>GHHHHHHHHHHSSGHIEGRHMRVLFVSSPGIGHLFPLIQLAWGFRTAGHDVLIAVAEHADRAAAAGLEVVDVAPDYSAVKVFEQVAKDNPRFAETVATRPAIDLEEWGVQIAAVNRPLVDGTMALVDDYRPDLVVYEQGATVGLLAADRAGVPAVQRNQSAWRTRGMHRSIASFLTDLMDKHQVSLPEPVATIESFPPSLLLEAEPEGWFMRWVPYGGGAVLGDRLPPVPARPEVAITMGTIELQAFGIGAVEPIIAAAGEVDADFVLALGDLDISPLGTLPRNVRAVGWTPLHTLLRTCTAVVHHGGGGTVMTAIDAGIPQLLAPDPRDQFQHTAREAVSRRGIGLVSTSDKVDADLLRRLIGDESLRTAAREVREEMVALPTPAET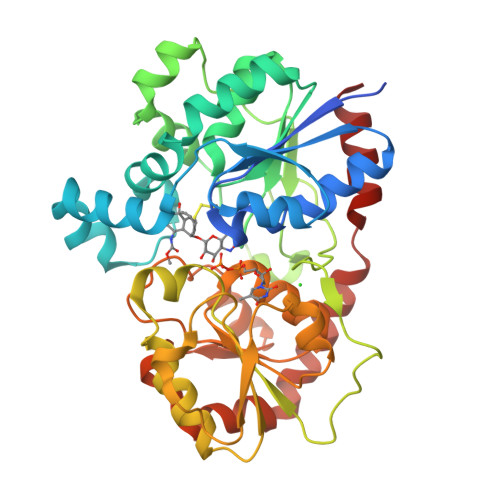VRRIVERISG[2x]> MFIYYKRTKQGSTEQWFVIGGKRIYLPTMTYVNE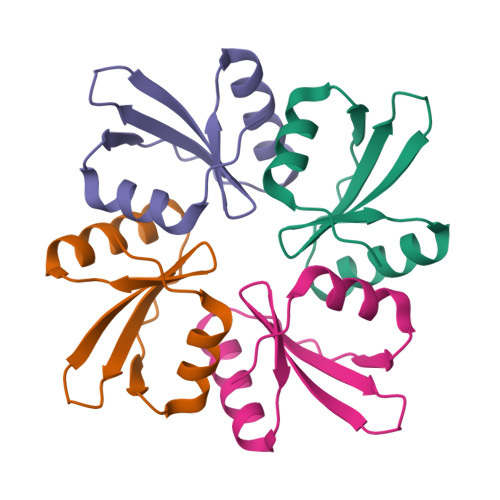ANDLIKRYGGNTNVTTYNHDNFGLKMMEAALPQVKV VcINDY is a Na+-dependent dicarboxylate transporter that imports TCA cycle intermediates across the inner membrane of Vibrio cholerae. The VcINDY protein is a homodimer consisting of a scaffold domain and a transport domain. Substrate transport of VcINDY is driven by the inwardly-directed Na+ gradient, with dicarboxylate import coupled to the co-transport of three sodium ions. Here, using a combination of cryo-EM structure determination, succinate binding and site-directed cysteine alkylation assays, we demonstrate that the VcINDY protein couples sodium- and substrate-binding via a previously unseen cooperative mechanism by conformational selection.

VcINDY was therefore purified in the presence of 100 mM Ch+ as the only monovalent cation. Unlike the VcINDY map in 300 mM Na+ for which 3D classification converged to a single map, the VcINDY-choline dataset yielded four distinct classes at a resolution range of 3.6—4.4 Å resolution. The 3D class with the highest resolution was further refined to 3.23 Å resolution. Whereas the overall fold of the protein in Ch+ remains the same, Na+ densities within the Na1 and Na2 clamshells are totally absent. While the VcINDY Ci-apo state overall structure is similar to those in the 300 mM Na+ (r.m.s.d of 0.672 Å), the model exhibited significant changes near the Na1 and N2 sites. The tip of HPin and the L10a-b loop have moved away from the Na1 and Na2 sites, respectively, with the carbonyls of Ala376 and Ala420, and the side chain of Asn378 also rotated away from the Na2 site. Notably, HPinb near the Na1 site and TM10b near the Na2 site and their connecting loops showed marked decreased density in the cryo-EM map, corresponding to the increased flexibility of these regions. In contrast, in the Ci-apo state the NMR-style analysis clearly illustrated the structural heterogeneity near the Na1 and Na2 sites. Instead of converging to one structure, the simulated annealing resulted in an ensemble of structures, with the greatest variations occurring in the HPinb and TM10b regions. As the 3.23 Å apo map imposes C2 symmetry on one of four classes of particles in ChCl, and all four classes are different, the degree of flexibility of these helices in the Ci-apo state is likely to be even greater. Such helix flexibility results from the absence of Na+ interactions with residues in the clamshells and with the dipoles of HPinb and TM10b.

>REWFLHRNSLIVLADVALFLALYHFLPFEHNVVLGISMLAFIAVLWLTEALHVTVTAILVPVMAVFFGIFETQAALNNFANSIIFLFLGGFALAAAMHHQGLDKVIADKVLAMAQGKMSVAVFMLFGVTALLSMWISNTATAAMMLPLVLGVLSKVDADKQRSTYVFVLLGVAYSASIGGIATLVGSPPNAIAAAEVGLSFTDWMKFGLPTAMMMLPMAIAILYFLLKPTLNGMFELDRAPVNWDKGKVVTLGIFGLTVFLWIFSSPINAALGGFKSFDTLVALGAILMLSFARVVHWKEIQKTADWGVLLLFGGGLCLSNVLKQTGTSVFLANALSDMVSHMGIFVVILVVATFVVFLTEFASNTASAALLIPVFATVAEAFGMSPVLLSVLIAVAASCAFMLPVATPPNAIVFASGHIKQSEMMRVGLYLNIACIGLLTAIAMLFWQ[2x]> NDPGKMLKDAIDKQVAGALVAGTTTSTHSVATDSTPALQAA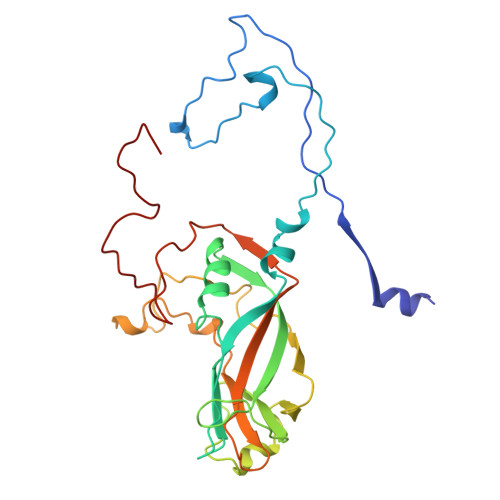ETGATSTARDESMIETRTIVPTHGIHETSVESFFGRSSLVGMPLLATGTSITHWRIDFREFVQLRAKMSWFTYMRFDVEFTIIATSSTGQNVTTEQHTTYQVMYVPPGAPVPSNQDSFQWQSGCNPSVFADTDGPPAQFSVPFMSSANAYSTVYDGYARFMDTDPDRYGILPSNFLGFMYFRTLEDAAHQVRFRIYAKIKHTSCWIPRAPRQAPYKKRYNLVFSGDSDRICSNRASLTSY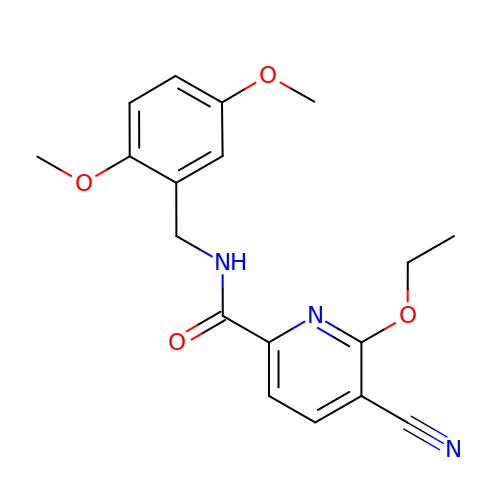5-CYANO-N-(2,5-DIMETHOXYBENZYL)-6-ETHOXYPYRIDINE-2-CARBOXAMIDE | C18 H19 N3 O4 | VEGKZYFYGCWXMN-UHFFFAOYSA-N hydroxy(3-{4-[(isoquinolin-5-yl)sulfonyl]piperazine-1-carbonyl}phenyl)oxoammonium 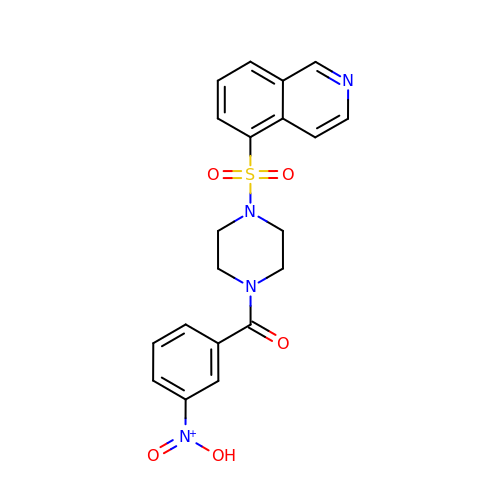| C20 H19 N4 O5 S | JQYQEKDPLZLZII-UHFFFAOYSA-N>KLAVAVVCSSNMNRSMEAHNFLAKKGFNVRSYGTGERVKLPGMAFDKPNVYEFGTKYEDIYRDLESKDKEFYTQNGLLHMLDRNRRIKKCPERFQDTKEQFDIIVTVEERVYDLVVMHMESMESVDNRPVHVLNVDVVDNAEDALMGAFVIT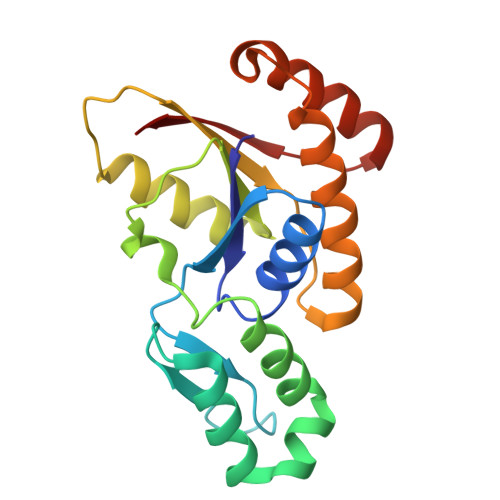DMINMMAKSTDLDNDIDELIQEFEERRKRVILHSVLFY[4x]>MPLLDSFKVDHTKMNAPAVRIAKTMLTPKGDNITVFDLRFCIPNKEILSPKGIHTLEHLFAGFMRDHLNGDSIEIIDISPMGCRTGFYMSLIGTPNEQKVSEAWLASMQDVLGVQDQASIPELNIYQCGSYTEHSLEDAHEIAKNVIARGIGVNKNEDLSLDNSLLK[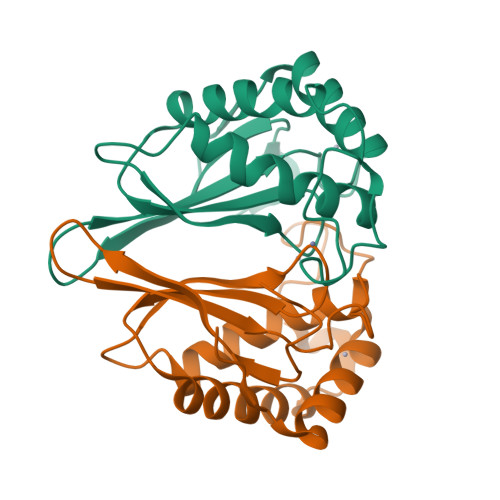4x]ChtII is a GH18 chitinase and possesses the greatest number of catalytic domains and chitin-binding domains in this family. Here we report the catalytic properties and the crystal structures of the catalytic domains of OfChtII, the ChtII derived from the Asian corn borer O. furnacalis. Analyzing the domain structure of the predicted protein with the SMART tool revealed that OfChtII contains five GH18 domains and seven CBM14-type chitin-binding modules (CBMs). The other two GH18 domains (C1 and C2) are predicted to be catalytically active (CAD).

The crystal of OfChtII-C1 was obtained by vapor diffusion, and the structure was determined using X-ray diffraction data at a resolution of 1.78 Å. The crystal belonged to space group P41212, and each asymmetric unit contained a single molecule. According to the structural characteristics, OfChtII-C1 could be divided into two distinct domains: a core domain and an insertion domain (CID). The core domain (residues 1613–1855 and 1940–1988, where the amino acid residues are numbered based on the full-length protein) is a classic (β/α)8 barrel with eight β-strands (β1–β8) tethered by eight α-helices (α1–α8). The CID (residues 1856–1939), which is composed of six antiparallel β-strands flanked by two short α-helices, is located between β7 and α7. The catalytic signature motif of GH18 chitinases, DXDXE (Asp1729–Glu1733), is located between β4 and α4. A long substrate-binding cleft, which comprises a series of conservative aromatic residues (Trp1621, Tyr1624, Trp1663, Trp1691, Trp1809, and Trp1961), is observed on the surface of OfChtII-C1. A conserved tryptophan on the surface of OfChtII-C1 was rotated 28.3° closer to the catalytic residue Glu1733 compared with the corresponding residue in OfChtII-C2, which could make the substrate more accessible to the catalytic residues. SmChiC lacks the α+β insertion domain, which is responsible for forming one “wall” of the substrate-binding cleft of OfChtII-C1.

> SLLNSRYKLVCYYTNWSWYRPGIGKYSPEDIDPSLCTHIVYGFAVLGNDGLMTAHDTWSDYDNRFYERVVEYKRYGIKVSLALGGWNDSAGDKYSKLVNDPAARAKFVQHAVAFLEKYGFDGLDLDWEYPKCWQVDCSKGPDSDKQGFADLVHELSAVLKPKGLLLSAAVSPNKMVIDAGYDVPVLARLLDWIAVMTYDYHGQWDKKTGHVAPLYYHPDDDTTYFNANYTIHYWMEKGTPASKIVMGMPMYGQSFTIENRGIHGLNIPVSDGGEPGEYTRAKGFLAYYEICDRIRNSGWTVVKDPYQRMGPYAYKGNQWVSFDDVEIIKKKVNFIKSLNLGGGMIWALDLDDYRNRCGQGKHPLLNAIKTELLNPKI[(3R,4S)-4-(thiophen-3-yl)pyrrolidin-3-yl]methanol 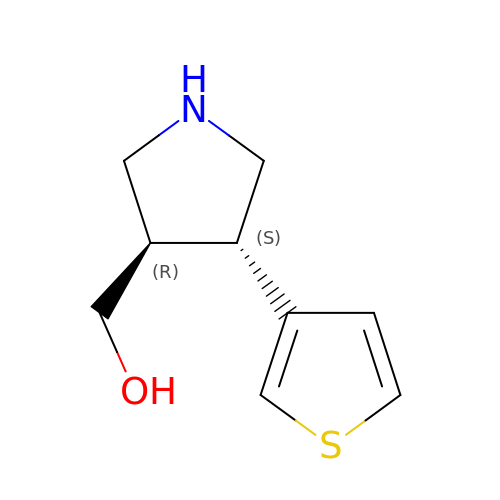| C9 H13 N O S | SWXORFHOLPJLTG-RKDXNWHRSA-N>[3x]MGSSHHHHHHSQDPVVEKEKSLSESDSSGYTGTFDI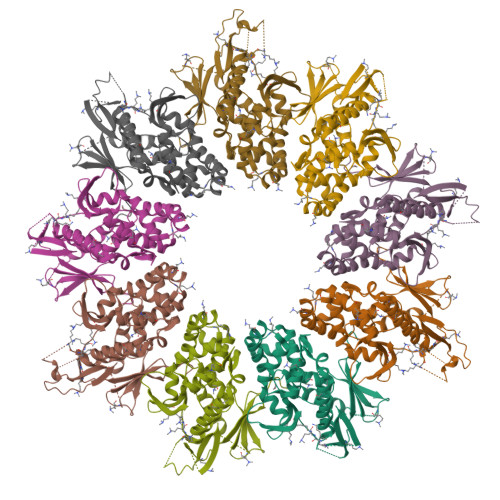DNSHDSSLAMIENLDAISSETVPLILLFAENKINANDMEGLIERIRSQFFIDYGVRLPTILYRTSNELKVDDIVLLINEVRADSFNIYFDKVCITDENGDIDALGIPVVSTSYNERVISWVDVSYTENLTNIDAKIKSAQDEFYHQLSQALLNNINEIFGIQETKNMLDQFENRYPDLLKEVFRHVTIQRISEVLQRLLGENISVRNLKLIMESLALWAPREKDVITLVEHVRASLSRYICSKIAVSGEIKVVMLSGYIEDAIRKGIRQTSGGSFLNMDIEVSDEVMETLAHALRELRNAKKNFVLLVSVDIRRFVKRLIDNRFKSILVISYAEIDEAYTINVLKTI> YFPPPAAKEDFLGCLVKEIPPRLLYAKSSPAYPSVLGQTIRNSRWSSPDNVKPLYIITPTQVSHIQSAVVCGRRHSVRIRVRSGGHDYEGLSYRSLQPETFAVVDLNKMRAVWVDGKARTAWVDSGAQLGELYYAIYKASPTLAFPAGVCPTIGVGGNFAGGGFGMLLRKYGIAAENVIDVKLVDANGKLHDKKSMGDDHFWAVRGGGGESFGIVVAWQVK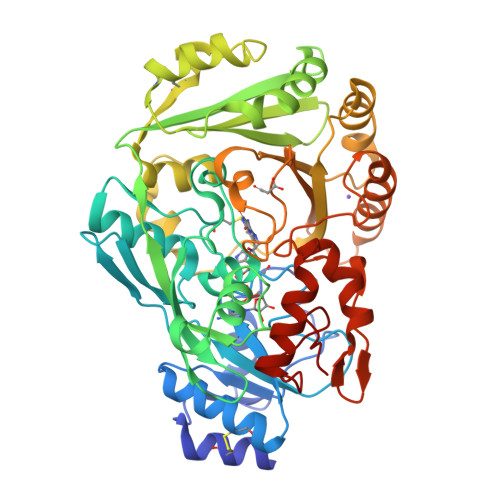LLPVPPTVTIFKISKTVSEGAVDIINKWQVVAPQLPADLMIRIIAQGPKATFEAMYLGTCKTLTPLMSSKFPELGMNPSHCNEMSWIQSIPFVHLGHRDALEDDLLNRQNSFKPFAEYKSDYVYQPFPKTVWEQILNTWLVKPGAGIMIFDPYGATISATPESATPFPHRKGVLFNIQYVNYWFAPGAAAAPLSWSKDIYNYMEPYVSKNPRQAYANYRDIDLGRNEVVNDVSTYASGKVWGQKYFKGNFERLAITKGKVDPTDYFRNEQSIPPLIKKY> GSKEDSVEAVGAQLKVYHQQYQDKSREYDQLYE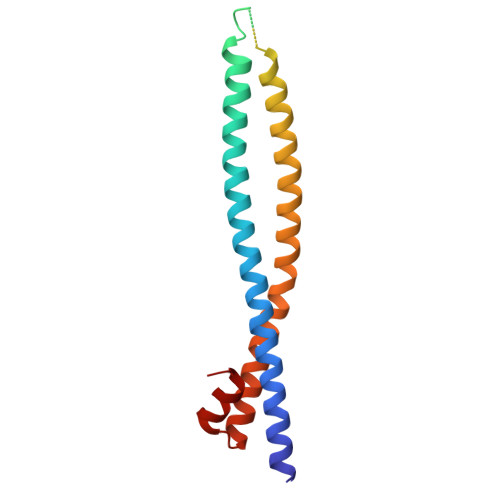EYTRTSQELQMKRTAIEAFNETIKIFEEQGQTQEKCSKEYLERFRREGNEKEMQRILLNSERLKSRIAEIHESRTKLEQQLRAQASDNREIDKRMNSLKPDLMQLRKIRDQYLVWLTQKGARQKKINEWLGI>[2x]MSYASLSVKDLTSLVSRSGTGSSSSLKPPGQTRPVKVIPLQHPDTSNEARPPSIPFDDIFSGWTAKIKRMRLVDWIDTLFPCFRWIRTYRWSEYFKLDLMAGITVGIMLVPQAMSYAKLAGLPPIYGLYSSFVPVFVYAIFGSSRQLAIGPVALVSLLVSNALGGIADTNEELHIELAILLALLVGILECIMGLLRLGWLIRFISHSVISGFTSASAIVIGLSQIKYFLGYSIARSSKIVPIVESIIAGADKFQWPPFVMGSLILVILQVMKHVGKAKKELQFLRAAAPLTGIVLGTTIAKVFHPPSISLVGEIPQGLPTFSFPRSFDHAKTLLPTSALITGVAILESVGIAKALAAKNRYELDSNSELFGLGVANILGSLFSAYPATGSFSRSAVNNESEAKTGLSGLITGIIIGCSLLFLTPMFKYIPQCALAAIVISAVSGLVDYDEAIFLWRVDKRDFSLWTITSTITLFFGIEIGVLVGVGFSLAFVIHESANPHIAVLGRLPGTTVYRNIKQYPEAYTYNGIVIVRIDSPIYFANISYIKDRLREYEVAVDKYTNRGLEVDRINFVILEMSPVTHIDSSAVEALKELYQEYKTRDIQLAISNPNKDVHLTIARSGMVELVGKEWFFVRVHDAVQVCLQYVQSSNLEDKHLSFTRRYGGSNNNSSSSNALLKEPLLSVEK

Higher plants have evolved a family of SO42− transporters, SULTRs, that mediate absorption of SO42− from the soil and its distribution to the entire organism. AtSULTR4;1 forms a homodimer and has a structural fold typical of the SLC26 family of anion transporters. We visualize the structure of AtSULTR4;1 with bound SO42− and demonstrate that AtSULTR4;1 is an H+/SO42− symporter. We show that H+ transport is likely mediated by a glutamate residue (Glu347) highly conserved among the plant SULTR family and that the cytosolic STAS domain modulates the transport process.

We determined the structure of AtSULTR4;1 at pH 6.0 in the presence of SO42− by cryo-electron microscopy (cryo-EM) to an overall resolution of 2.8 Å. The final model consists of residues 70–644. The STAS domains are swapped between the neighboring subunits. The SO42− is located between the N-termini of TM3 and TM10, and is coordinated by side-chain and backbone atoms entirely from the core domain. Sidechain hydroxyls of Tyr116 and Ser392 are within hydrogen bond distance to SO42−; and so are backbone amides of Ala153, Phe391, and Ser392. A conserved Arg393 from TM10 is ~5 Å away and although it does not make direct contact with the SO42−, it likely provides the positive electrostatic potential for the binding pocket. The helix dipoles of TM3 and TM10 are oriented with their positive ends pointing to the bound SO42−, providing the positive electrostatic potential to the bound SO42−. A negatively charged residue, Glu347 on TM8, is ~7 Å away from the bound SO42−. In the current structure of AtSULTR4;1, both the bound SO42− and the putative proton sensing site Glu347 are solvent accessible only from the intracellular side, and thus the current structure is in an inward-facing conformation. However, in our structure, the N-terminus (residues 1–69) is not resolved and we do not observe densities at the corresponding position on the STAS domain. Although most of the dimer interface is contributed by the interactions between the two STAS domains, the domain-swapped arrangement in dimerization leads to the interaction of each STAS domain with the core and gate domains of the neighboring subunit.Sirtuins generally catalyze the deacylation of modified lysine residues in protein substrates coupled with the breakdown of NAD+ into nicotinamide (NAM) and 2'-O-acyl-ADP-ribose. To address this, we developed an engineered hSIRT1 (mini-hSIRT1) that is biochemically equivalent to the full-length enzyme with respect to basal catalytic activity and activation by STACs. Mini-hSIRT1 comprises a catalytic domain that assumes a Rossmann-fold large lobe and a zinc-binding small lobe common to all sirtuins, an N-terminal three-helical bundle encompassing the SBD and a C-terminal β-hairpin CTR peptide18.

In the quaternary complex structure, the Ac-p53 peptide and carbaNAD bind to the active site cleft between the large and small lobes. Ac-p53 adopts an extended conformation, similar to the backbone-mediated β-strand like interactions observed in many Sirtuin/Ac-peptide complexes. The main chain amide groups of Ac-p53 form hydrogen bonds with those of the residues Gly415 and Glu416 from the small lobe and those of the residues Lys444 and Arg446 from the large lobe. The hydrogen bonds between the amide of the peptide +1 position and that of Arg446 render a potential interaction between the side chain and a bulky and hydrophobic +1 residue, which might be important in STAC-mediated hSIRT1 activation. The acetyl-lysine side chain inserts into a hydrophobic cavity lined by Phe414, Leu418 and Val445. The acetyl group is sandwiched between His363 and Phe297, with the ɛ-N of the acetyl-lysine hydrogen bonded with the carbonyl oxygen of Val412, which maintains the orientation and the extended conformation of the acetyl-lysine side chain. CarbaNAD also makes multipoint contacts with hSIRT1, most of which are similar to those observed in reported Sirtuin/NAD+ strucutres1931. Similar to SIRT3, binding of substrates or the active-site inhibitor leads to domain closure, bringing the small and large lobes together. Comparison of the three structures shows that the locations of the N-terminal SBD domain relative to the catalytic core are divergent among the three structures, likely to be impacted by different crystal packings. (2) How does the STAC binding in the N-terminal SBD enhance the substrate binding at the active site, which is not obvious from the comparison of current structures of Mini-SIRT1/1 and Mini-SIRT1/1/ p53 7-mer/CarbaNAD?

> GPYTFVQQHLMIGTDPRTILKDLLPETIPPPELDDMTLWQIVINILSEPPKRKKRKDINTIEDAVKLLQECKKIIVLTGAGVSVSCGIPDFRSRDGIYARLAVDFPDLPDPQAMFDIEYFRKDPRPFFKFAKEIYPGQFQPSLCHKFIALSDKEGKLLRNYTQNIDTLEQVAGIQRIIQCHGSFATASCLICKYKVDCEAVRGDIFNQVVPRCPRCPADEPLAIMKPEIVFFGENLPEQFHRAMKYDKDEVDLLIVIGSSLKVRPVALIPSSIPHEVPQILINREPLPHLHFDVELLGDCDVIINELCHRLGGEYAKLCCNPVGGGSGGGSQYLFLPPNRYIFHGAEVYSDSEDDV;> RHKKLLF11-[(2~{R})-2-[(2-pyridin-3-ylquinazolin-4-yl)amino]-2,3-dihydro-1~{H}-inden-5-yl]undec-10-ynoic acid | C33 H34 N4 O2 | 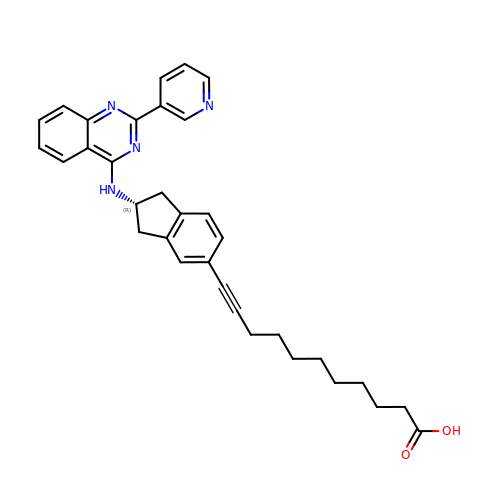OOVVDXXXFLHSBX-MUUNZHRXSA-N> GP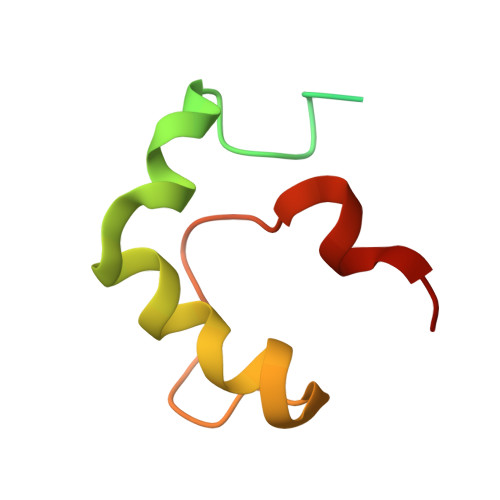HMGSPEFDGTLVRIWMPDGAPAYTADTEAEDPKVYEDEGVKRQWQSFLEKGRFEGGMPEVPPRREWCVWDF> GHMTASPRAPHQEHVLGEPTLEGLAHYIREKNVRRILVLVGAGASVAAGIPDFRSPDTGIYANLGKYNLEDPTDAFSLTLLREKPEIFYSIARELNLWPGHFQPTAVHHFIRLLQDEGRLLRCCTQNIDGLEKAAGVSPELLVEAHGSFAAAACIECHTPFSIEQNYLEAMSGTVSRCSTCGGIVKPNVVFFGENLPDAFFDALHHDAPIAELVIIIGTSMQVHPFALLPCVVPKSVPRVVMNRERVGGLLFRFASTSSSSDGYGQYGDYHAHPDVCRDVLFRGDCQENVVT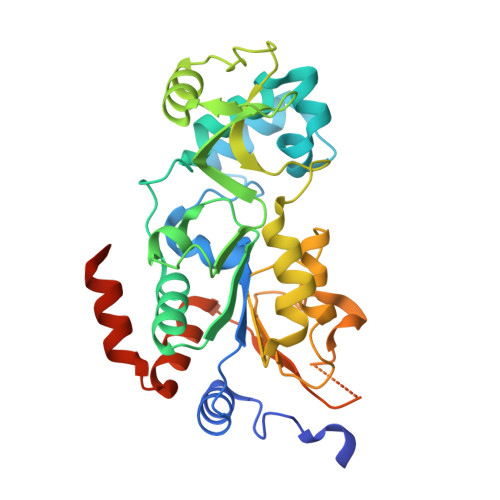LAEYLGLSEALAKRMRLSDAAPATAQRAPNET>[9x]MADISRAEVA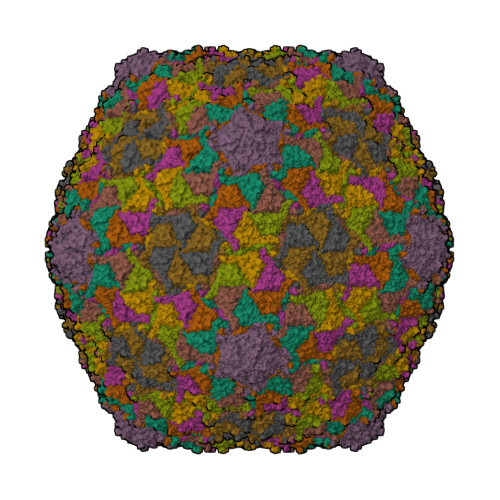TLIQEAYSDTLLAAAKQGSTVLSAFQNVNMGTKTTHLPVLATLPEAGWVGESATEPEGVIPTSKVTWANRTLVAEEVAVIIPVPEAVIDDATVAILTEVAEQGGQAIGKKLDQAVIFGIDKPASWVSPALVPAAVAAGQAIAHVSGVANEFDLVGASNKVAEKVALAGWAPDTLLSSLALRYQVANVRDADGNLAFRDGSFLGFNTHFNRNGAWAPTSAVGVIADSSRVKIGVRQDITVKFLDQATLGTGENQINLAERDMVALRLKARFAYVLGVSATSVGANQTPVGVVTPDVTA>[2x]MPSQAALLIGDIVHARAEWEALSSLVTLKEFPEGGREKFLENCKSGQYDDVIAIYRSNISTKHTGPFDRELISALPKSVKYICHNGAGY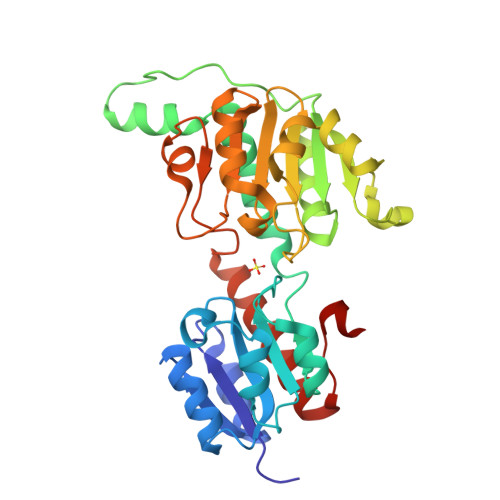DNIDVDAATEAGIAISSTPIAVNNATADVAIFLMIGALRQAYVPITAIRAGEWHGKTTLGHDPNGKTLGILGMGGIGREVARRARAFGMNIIYHNRNKLPPELEDGAKYVSFDELLAQSDVFSLNLALNASTRHIIGEKELAKMKDGVVIVNTARGALIDEKALVRALESGKVASVGLDVYENEPQVEPGLLNNPRAMLLPHIGTMTYETQKEMELLVLNNLRSAIEKGELLTQVPEQKKR>[2x]MVKIV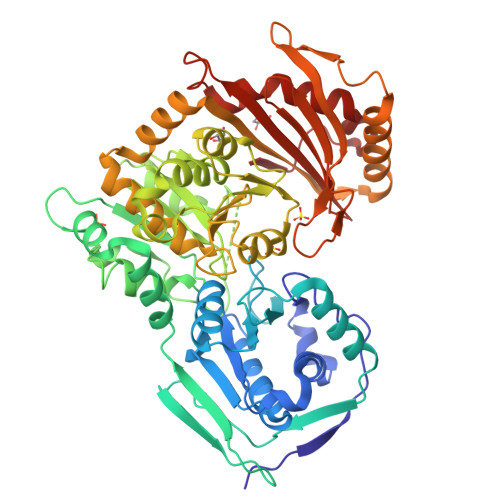TVKTQAYQDQKPGTSGLRKRVKVFQSSANYAENFIQSIISTVEPAQRQEATLVVGGDGRFYMKEAIQLIARIAAANGIGRLVIGQNGILSTPAVSCIIRKIKAIGGIILTASHNPRGPNGDFGIKFNISNGGPAPEAITDKIFQISKTIEEYAVCPDLKVDLGVLGKQQFDLENKFKPFTVEIVDSVEAYATMLRSIFDFSALKELLSGPNRLKIRIDAMHGVVGPYVKKILCEELGAPANSAVNCVPLEDFGGHHPDPNLTYAADLVETMKSGEHDFGAAFDGDGDRNMILGKHGFFVNPSDSVAVIAANIFSIPYFQQTGVRGFARSMPTSGALDRVASATKIALYETPTGWKFFGNLMDASKLSLCGEESFGTGSDHIREKDGLWAVLAWLSILATRKQSVEDILKDHWQKYGRNFFTRYDYEEVEAEGANKMMKDLEALMFDRSFVGKQFSANDKVYTVEKADNFEYSDPVDGSISRNQGLRLIFTDGSRIVFRLSGTGSAGATIRLYIDSYEKDVAKINQDPQVMLAPLISIALKVSQLQERTGRTAPTVIT>[6x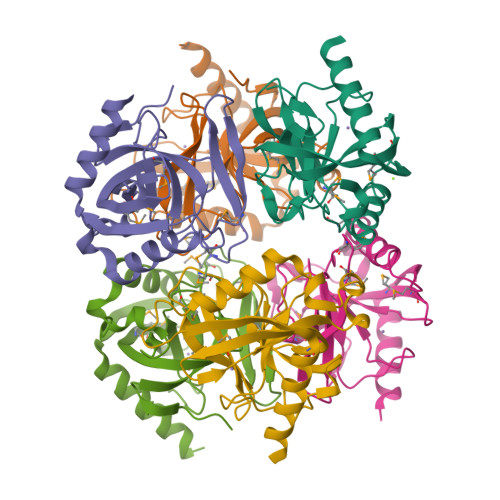]SYVMTFLVSAGKGIDDFNVIIEIPANGGEVKYEYDKELGFLTVDRFMPTSMRYPCNYGFVPSTLAQDGDPLDVLVLTPVPVQPGVLMRVRALGIMKMEDEAGEDSKVLAVPVVKACRAYEAIQSLKDISSLLLDAISHFFERYKDLEPNKWAKVKGWEDKEAAKKEFEASIVRFKEKK>[2x]MSSAEEKLFMKALKEKFEESPEEKYTKFYIFGGWKQSERKKEFKEWADKIVEERGVPHYNPDIGVPLGQRKLMSYQVSGTDVFVEGDDLTFVNNAAMQQMWDDIRRTVIVGMDTAHRVLERRLGKEVTPETINEYMETLNHALPGGAVVQEHMVEIHPGLTWDCYAKIITGDLELADEIDDKFLIDIEKLFPEEQAEQLIKAIGNRTYQVCRMPTIVGHVCDGATMYRWAAMQIAMSFICAYKIAAGEAAVSDFAFASKHAEVINMGEMLPARRARGENEPGGVPFGVLADCVQTMRKYPDDPAKVALEVIAAGAMLYDQIWLGSYMSGGVGFTQYATAVYPDNILDDYVYYGLEYVEDKYGIAEAEPSMDVVKDVATEVTLYGLEQYERYPAAMETHFGGSQRAAVCAAAAGCSTAFATGHAQAGLNGWYLSQILHKEGQGRLGFYGYALQDQCGAANSLSVRSDEGLPLELRGPNYPNYAMNVGHLGEYAGIVQAAHAARGDAFCVHPVIKVAFADENLVFDFTEPRKEFAKGALREFEPAGERDLIVPAE;>MAREAKDTVDLYDDRGNCVAEEVPIEVLSPMRNEAIQSIVNDIKRTVAVDLEGIENALQNATVGGKGMKIPGREMDVDIVDNAEAIADEIEKMIRVYQDDDTNVEPMYDGKRLLVQLPSERVKVM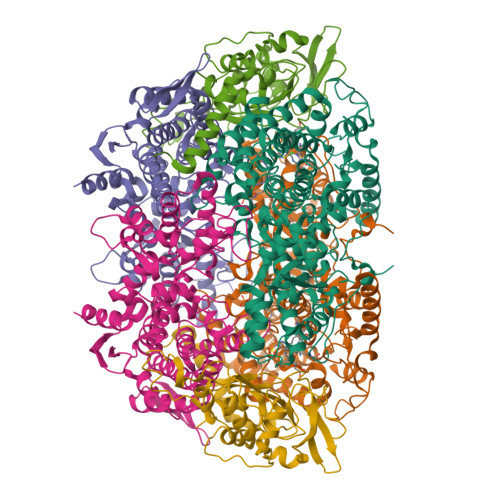ADPYSGTLQAGMAVVHAIIDVCEVDMWDANMVKAAVFGRYPQTIDYFGGNVASMLDVPMKQEGVGYALRNIMVNHIVAATRKNTMQAVCLAATLQQTAMFEMGDALGPFERLHLLGYAYQGLNADNMVYDIVKKHGKEGTVGTVVREVVERALEDGVIEVKEELPSFKVYKANDMDLWNAYAAAGLVAAVMVNQGAARAAQGVSATILYYNDLLEYETGLPGVDFGRAEGTAVGFSFFSHSIYGGGGPGIFHGNHIVTRHSKGFAIPPVAAAMALDAGTQMFSPEVTSKLIGDVFGEIDEFREPMKYITEAAAEEAKR[2x];>MAEKAQFYYPGETDVAENRRKYMNPNYELKKLREIPDEDIVRLMGHREPGEEYPSVHPPLEEMEEPECPIRELVEPTEGAKAGDRIRYIQFTDSVYFAPIHPYIRARMYMWRYRGVDTGSLSGRQIIEVRERDLEKIAKELLETEIFDPARSGVRGATVHGHALRLDENGLMLHALRRYRLNEETGEVEYVKDQVGIELDEPIPVGAPADEDDLKERTTIYRIDGTPYREDEELLQVVQRIHELRTLAGYRPEEAEGK[2x]>[4x]MSAKAISEQTGKELLYKFICTTSAIQNRFKYARVTPDTDWARLLQDHPWLLSQNLVVKPDQLIKRRGKLGLVGVNLTLDGVKSWLKPRLGQEATVGKATGFLKNFLIEPFVPHSQAEEFYVCIYATREGDYVLFHHEGGVDVGDVDAKAQKLLVGVDEKLNPEDIKKHLLVHAPEDKKEILASFISGLFNFYEDLYFTYLEINPLVVTKDGVYVLDLAAKVDATADYICKVKWGDIEFPPPFGREAYPEEAYIADLDAKSGASLKLTLLNPKGRIWTMVAGGGASVVYSDTICDLGGVNELANYGEYSGAPSEQQTYDYAKTILSLMTREKHPDGKILIIGGSIANFTNVAATFKGIVRAIRDYQGPLKEHEVTIFVRRGGPNYQEGLRVMGEVGKTTGIPIHVFGTETHMTAIVGMALGHRPIPNQPPTAAHTANFLLNASGSTSTPAPSRTASFSESRADEVAPAKKAKPAMPQDSVPSPRSLQGKSTTLFSRHTKAIVWGMQTRAVQGMLDFDYVCSRDEPSVAAMVYPFTGDHKQKFYWGHKEILIPVFKNMADAMRKHPEVDVLINFASLRSAYDSTMETMNYAQIRTIAIIAQGIPEALTRKLIKKADQKGVTIIGPATVGGIKPGCFKIGNTGGMLDNILASKLYRPGSVAYVSRSGGMSNELNNIISRTTDGVYEGVAIGGDRYPGSTFMDHVLRYQDTPGVKMIVVLGEIGGTEEYKICRGIKEGRLTKPIVCWCIGTCATMFSSEVQFGHAGACANQASETAVAKNQALKEAGVFVPRSFDELGEIIQSVYEDLVANGVIVPAQEVPPPTVPMDYSWARELGLIRKPASFMTSICDERGQELIYAGMPITEVFKEEMGIGGVLGLLWFQKRLPKYSCQFIEMCLMVTADHGPAVSGAHNTIICARAGKDLVSSLTSGLLTIGDRFGGALDAAAKMFSKAFDSGIIPMEFVNKMKKEGKLIMGIGHRVKSINNPDMRVQILK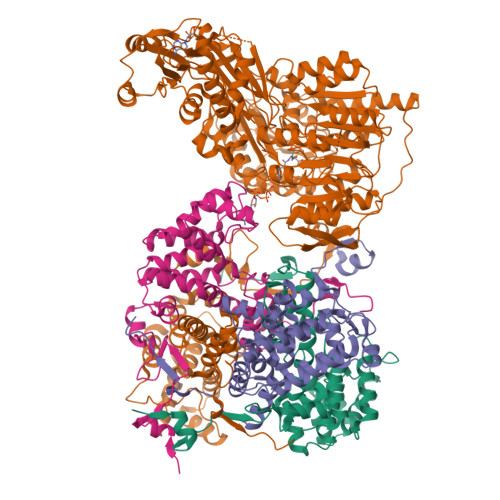DYVRQHFPATPLLDYALEVEKITTSKKPNLILNVDGLIGVAFVDMLRNCGSFTREEADEYIDIGALNGIFVLGRSMGFIGHYLDQKRLKQGLYRHPWDDISYVLPEHMSM>[2x]MGPSPPGNLRVTDVTSTSVTLSWWPEIVPLHGYRVEYREAGGEWKEVTVIDRAPEYTVTGL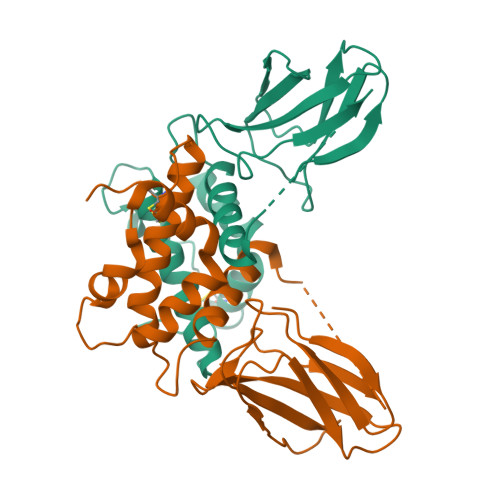KPGTEYEFRVRAVSGALYFNASSVSVTTGGGSGGSGGDGGGSGDGGSGSGSGGGGDSGSSGGSGSGGGSNTQAERSIIGMIDMFHKYTRRDDKIDKPSLLTMMKENFPNFLSACDKKGTNYLADVFEKKDKNEDKKIDFSEFLSLLGDIATDYHKQSHGAAPCSGGSQKLAAALEHHHHHH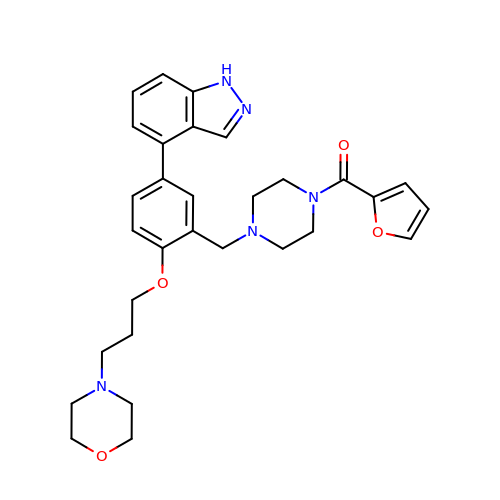(furan-2-yl)[4-({(5P)-5-(1H-indazol-4-yl)-2-[3-(morpholin-4-yl)propoxy]phenyl}methyl)piperazin-1-yl]methanone | C30 H35 N5 O4 | SAFWOFNFKMPJAO-UHFFFAOYSA-N2,6-dichloro-N-(2-oxo-2,5-dihydropyridin-4-yl)benzamide | 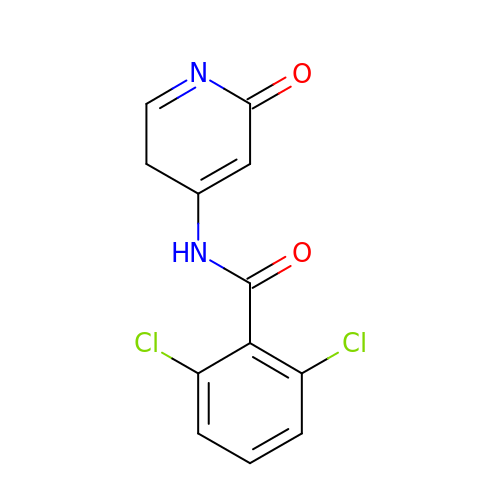C12 H8 Cl2 N2 O2 | HKIJJBMBTHKEPC-UHFFFAOYSA-N POGLUT1 is an inverting GT-B fold (CAZy GT Family 9018) glycosyltransferase and its EGF-like domain substrates sit in a cleft formed between the canonical N-terminal and C-terminal domains. Here we report the structure of human POGLUT1 in complexes with three different EGF-like domains and either UDP, a donor substrate analog or a slow substrate. The structures reveal the basis for POGLUT1’s ability to recognize diverse EGF-like domain substrates and for the requirement that they be folded. The three EGF-like domains studied are positioned almost identically in their respective complexes and 25–30% of their surface (740–830 Å2) is buried by POGLUT1.

In the POGLUT1/hEGF12/UDP complex, the presence of the Asp sidechain at the i + 2 position of hEGF12 further extends the interaction surface with Trp174. Among the EGF-like domains studied here, EGF(+) (C1ASNPC2) and hEGF12 (C1VSNPC2) do not possess a diserine-containing motif, while hF7EGF1 (C1ASSPC2) does. Of the EGF-like domains studied, hEGF12 and EGF(+) contain an asparagine residue at the Xb position (C1XaSNPC2) while hF7EGF1 contains a serine (C1XaSSPC2). In all cases, the asparagine and serine sidechains make a strong hydrogen bond to the backbone NH group of Gln240. In both the POGLUT1/hF7EGF1/UDP and POGLUT1/hEGF12/UDP complexes, the serine hydroxyl is found only in the gauche (−) rotamer where it is hydrogen bonded to the sidechain of the catalytic base and positioned for nucleophilic attack. To explore this further, we assayed hEGF12 and EGF(+), substrates lacking diserine, and found that they can both be readily xylosylated. The ability to xylosylate hEGF12, an EGF-like domain possessing the C1XaSNPC2 motif found in 36% of POGLUT1 substrates, shows that POGLUT1 has the potential to xylosylate many more EGF-like domains than previously thought.

> GSKWKVFIDQINRSLENYEPCSSQNCSCYHGVIEEDLTPFRGGISRKMMAEVVRRKLGTHYQITKNRLYRENDCMFPSRCSGVEHFILEVIGRLPDMEMVINVRDYPQVPKWMEPAIPVFSFSKTSEYHDIMYPAWTFWEGGPAVWPIYPTGLGRWDLFREDLVRSAAQWPWKKKNSTAYFRGSRTSPERDPLILLSRKNPKLVDAEYTKNQAWKSMKDTLGKPAAKDVHLVDHCKYKYLFNFRGVAASFRFKHLFLCGSLVFHVGDEWLEFFYPQLKPWVHYIPVKTDLSNVQELLQFVKANDDVAQEIAERGSQFIRNHLQMDDITCYWENLLSEYSKFLSYNVTRRKGYDQIIP;> GSDVNECVSNPCQNDATCLDQIGEFQCICMPGYEGVHCEVNT> MEQANPLRPDGESKGGVLAHLERLETQVSRSRKQSEELQSVQAQEGALGTKIHKLRRLRDELRAVVRHRRASVKACIANVEPNQTVEINEQEALEEKLENVKAILQAYHFTGLSGKLTSRGVCVCISTAFEGNLLDSYFVDLVIQ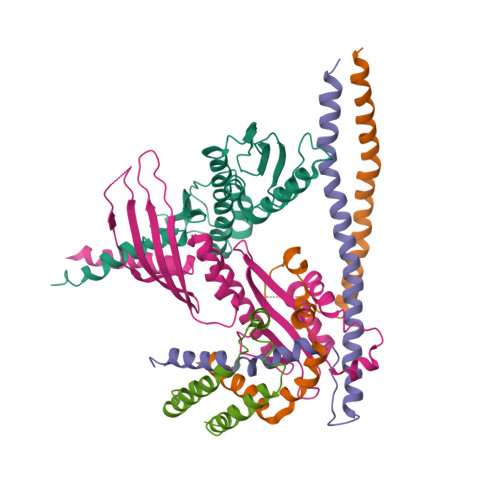KPLRIHHHSVPVFIPLEEIAAKYLQTNIQHFLFSLCEYLNAYSGRKYQADRLQSDFAALLTGPLQRNPLCNLLSFTYKLDPGGQSFPFCARLLYKDLTATLPTDVTVTCQGVEVLSTSWEEQRASHETLFCTKPLHQVFASFTRKGEKLDMSLVS;> MDAELAEVRALQAEIAALRRACEDPPAPWEEKSRVQKSFQAIHQFNLEGWKSSKDLKNQLGHLESELSFLSTLTGINIRNHSKQTEDLTSTEMTEKSIRKVLQRHRLSGNCHMVTFQLEFQILEIQNKERLSSAVTDLNIIMEPTECSELSEFVSRAEERKDLFMFFRSLHFFVEWFEYRKRTFKHLKEKYPDAVYLSEGPSSCSMGIRSASRPGFELVIVWRIQIDEDGKVFPKLDLLTKVPQRALELDKNRAIETAPLSFRTLVGLLGIEAALESLIKSLCAEENNENLYFQ;> MDLTNVSSLLNMERARDKANEEGLALLQEEIDKMVETTELMTGNIQSLKNKIQILASEVEEEEERVKQMHQINSSGVLSLPELSQKTLKAPTLQKEILALIPNQNALLKDLDILHNSSQMKSMSTFIEEAYKKLDAS;> MPVKRSLKLDGLLEENSFDPSKITRKKSVITYSPTTGTCQMSLFASPTSSEEQKHRNGLSNEKRKKLNHPSLTESKESTTKDNDEFMMLLSKVEKLSEEIMEIMQNLSSIQALEGSRELENLIGISCASHFLKREMQKTKELMTKVNKQKLFEKSTGLPHKASRHLDSYEFLKAILN;> MAPRGRRRPRPHRSEGARRSKNTLERTHSMKDKAGQKCKPIDVFDFPDNSDVSSIGRLGENEKDEETYETFDPPLHSTAIYADEEEFSKHCGLSLSSTPPGKEAKRSSDTSGNEASEIESVKISAKKPGRKLRPISDDSESIEESDTRRKVKSAEKISTQRHEVIRTTASSELSEKPAESVTSKKTGPLSAQPSVEKENLAIESQSKTQKKGKISHDKRKKSRSKAIGSDTSDIVHIWCPEGMKTSDIKELNIVLPEFEKTHLEHQQRIESKVCKAAIATFYVNVKEQFIKMLKESQMLTNLKRKNAKMISDIEKKRQRMIEVQDELLRLEPQLKQLQTKYDELKERKSSLRNAAYFLSNLKQLYQDYSDVQAQEPNVKETYDSSSLPALLFKARTLLGAESHLRNINHQLEKLLDQG Streptococcus pyogenes M1 GAS SF370 ORF Spy1604 encodes a putative GH38 α-mannosidase. We have shown that The S. pyogenes ORF spy1604 encodes an α−1,3 mannosidase that is active on disaccharides, some aryl glycosides and can also effectively deglycosylate human N-glycans in vitro. This, coupled to the presence of a gene encoding an N-acetyl glucosaminidase (Spy1600) on the operon (an enzyme known to break β−linked N-acetylglucosaminides) would suggest a role, in vivo, in the utilization of human glycan-derived carbohydrates as a nutrient source. Comparison of SpGH38 with Drosophila Golgi α−mannosidase II suggests a conserved domain architecture and catalytic centre in which diversification in the “leaving group” subsites accounts for the subtly different specificity.

Overall, the individual domains and architecture of SpGH38 are similar to both dGMII and bLAM, albeit different in spatial arrangement and intra-domain contacts, overlapping full length secondary structures with mean square deviations of 2.6 and 2.8 Å, respectively. Secondary structure matching of full length SpGH38 using SSM not surprisingly reveals the GH38 Drosophila α−mannosidase II as the top “hit” (Z score 9.8 with 664 residues aligning, r.m.s.d 2.6 Å). However, the structural divergence was significant enough to prevent either being used as a suitable molecular replacement model for SpGH38, even when shorter, more conserved, features were used. The α/β-domain features a distorted β-barrel core composed of primarily parallel strands, surrounded by eight helices of varying length and an appreciable amount of coil. As discussed, SpGH38 appears to exist as an elongated dimer. The SpGH38 dimer forms through an inter-digitation of the β−3 domain into the opening formed between α/β and β−2 domains of an adjacent molecule. A series of van der Waals' and hydrogen bonding interactions stabilize this intra-molecular connection involving hydrophobic residues Y574, V629, W764, Y766, F767 from the α/β and β−2 domains with F429, F433, P434, Y438, F474, Y476, L478, P479, F483, P486, and F488 of the β−3 domain which would be surface exposed in a monomeric state. This insertion of the β−3 domain effectively reduces the area of the putative Man5GlcNAc binding site in an adjacent molecule and introduces Y476, F483, R484, and Q431 which could putatively stabilize GlcNAc and Man substituents thereby anchoring a high mannose substrate. One possible reason for this may be the insertion of the β−1 domain into the active centre of the dimer mate in the crystal forms observed here. In particular, Arg484 from this loop stacks with W764 discussed above, thus reducing accessibility to the +1 subsite in-crystal.

>MGSSHHHHHHSSGLEVLFQGPAMATKKVHIISHSHWDREWYMAYEQHHMRLINLIDDLLEVFQTDPDFHSFHLDGQTIILDDYLKVRPEREPEIRQAIASGKLRIGPFYILQDDFLTSSESNVRNMLIGKEDCDRWGASVPLGYFPDTFGNMGQTPQLMLKAGLQAAAFGRGIRPTGFNNQVDTSEKYSSQFSEISWQGPDNSRILGLLFANWYSNGNEIPTTEAEARLFWDKKLADAERFASTKHLLMMNGCDHQPVQLDVTKAIALANQLYPDYEFVHSCFEDYLADLADDLPENLSTVQGEITSQETDGWYTLANTASARIYLKQANTRVSRQLENITEPLAAMAYEVTSTYPHDQLRYAWKTLMQNHPHDSICGCSVDSVHREMMTRFEKAYEVGHYLAKEAAKQIADAIDTRDFPMDSQPFVLFNTSGHSKTSVAELSLTWKKYHFGQRFPKEVYQEAQEYLARLSQSFQIIDTSGQVRPEAEILGTSIAFDYDLPKRSFREPYFAIKVRLRLPITLPAMSWKTLALKLGNETTPSETVSLYDDSNQCLENGFLKVMIQTDGRLTITDKQSGLIYQDLLRFEDCGDIGNEYISRQPNHDQPFYADQGTIKLNIISNTAQVAELEIQQTFAIPISADKLLQAEMEAVIDITERQARRSQEKAELTLTTLIRMEKNNPRLQFTTRFDNQMTNHRLRVLFPTHLKTDHHLADSIFETVKRPNHPDATFWKNPSNPQHQECFVSLFDGENGVTIGNYGLNEYEILPDTNTIAITLLRSVGEMGDWGYFPTPEAQCLGKHSLSYSFESITKQTQFASYWRAQEGQVPVITTQTNQHEGTLAAEYSYLTGTNDQVALTAFKRRLADNALITRSYNLSNDKTCDFSLSLPNYNAKVTNLLEKDSKQSTPSQLGKAEILTLAWKKQ[2x]> HHHHHHHMDITKVDTSG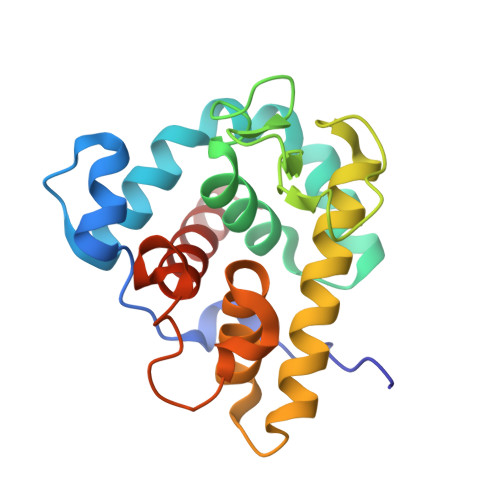ASEITARQDKLTLQGVDASHKLAEHDLVRMNKYKELITRVGQKHGLDPAIIAGIISRESRAGSALDHGWGDHGKGFGLMQVDKRYHKIVGAWDSEKHISQGTEILIEFIRRIQAKFPVWPKEHQLKGGISAYNAGDKNVRTYERMDVGTTGGDYSNDVVARSQWFKSQGY>[2x]MKPEVEQELAHILLTELLAYQFASPVRWIETQDVFLKDFNTERVVEIGPSPTLAGMAQRTLKNKYESYDAALSLHREILCYSKDAKEIYYTPDPSELAAKEEPAKEEAPAPTPAASAPAPAAAAPAPVAAAAPAAAAAEIADEPVKASLLLHVLVAHKLKKSLDSIPMSKTIKDLVGGKSTVQNEILGDLGKEFGTTPEKPEETPLEELAETFQDTFSGALGKQSSSLLSRLISSKMPGGFTITVARKYLQTRWGLPSGRQDGVLLVALSNEPAARLGSEADAKAFLDSMAQKYASIVGVDLSSAASASGAAGAGAAAGAAMIDAGALEEITKDHKVLARQQLQVLARYLKMDLDNGERKFLKEKDTVAELQAQLDYLNAELGEFFVNGVATSFSRKKARTFDSSWNWAKQSLLSLYFEIIHGVLKNVDREVVSEAINIMNRSNDALIKFMEYHISNTDETKGENYQLVKTLGEQLIENCKQVLDVDPVYKDVAKPTGPKTAIDKNGNITYSEEPREKVRKLSQYVQEMALGGPITKESQPTIEEDLTRVYKAISAQADKQDISSSTRVEFEKLYSDLMKFLESSKEIDPSQTTQLAGMDVEDA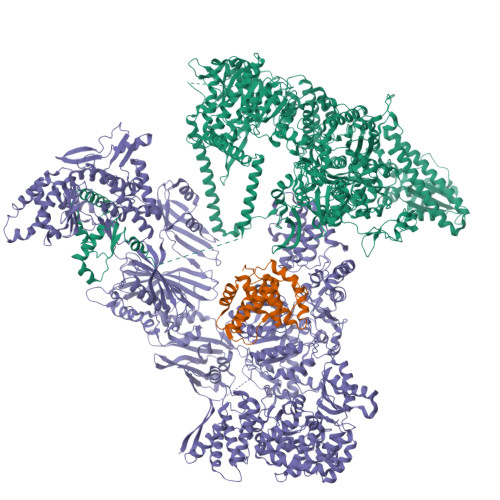LDKDSTKEVASLPNKSTISKTVSSTIPRETIPFLHLRKKTPAGDWKYDRQLSSLFLDGLEKAAFNGVTFKDKYVLITGAGKGSIGAEVLQGLLQGGAKVVVTTSRFSKQVTDYYQSIYAKYGAKGSTLIVVPFNQGSKQDVEALIEFIYDTEKNGGLGWDLDAIIPFAAIPEQGIELEHIDSKSEFAHRIMLTNILRMMGCVKKQKSARGIETRPAQVILPMSPNHGTFGGDGMYSESKLSLETLFNRWHSESWANQLTVCGAIIGWTRGTGLMSANNIIAEGIEKMGVRTFSQKEMAFNLLGLLTPEVVELCQKSPVMADLNGGLQFVPELKEFTAKLRKELVETSEVRKAVSIETALEHKVVNGNSADAAYAQVEIQPRANIQLDFPELKPYKQVKQIAPAELEGLLDLERVIVVTGFAEVGPWGSARTRWEMEAFGEFSLEGCVEMAWIMGFISYHNGNLKGRPYTGWVDSKTKEPVDDKDVKAKYETSILEHSGIRLIEPELFNGYNPEKKEMIQEVIVEEDLEPFEASKETAEQFKHQHGDKVDIFEIPETGEYSVKLLKGATLYIPKALRFDRLVAGQIPTGWNAKTYGISDDIISQVDPITLFVLVSVVEAFIASGITDPYEMYKYVHVSEVGNCSGSGMGGVSALRGMFKDRFKDEPVQNDILQESFINTMSAWVNMLLISSSGPIKTPVGACATSVESVDIGVETILSGKARICIVGGYDDFQEEGSFEFGNMKATSNTLEEFEHGRTPAEMSRPATTTRNGFMEAQGAGIQIIMQADLALKMGVPIYGIVAMAATATDKIGRSVPAPGKGILTTAREHHSSVKYASPNLNMKYRKRQLVTREAQIKDWVENELEALKLEAEEIPSEDQNEFLLERTREIHNEAESQLRAAQQQWGNDFYKRDPRIAPLRGALATYGLTIDDLGVASFHGTSTKANDKNESATINEMMKHLGRSEGNPVIGVFQKFLTGHPKGAAGAWMMNGALQILNSGIIPGNRNADNVDKILEQFEYVLYPSKTLKTDGVRAVSITSFGFGQKGGQAIVVHPDYLYGAITEDRYNEYVAKVSAREKSAYKFFHNGMIYNKLFVSKEHAPYTDELEEDVYLDPLARVSKDKKSGSLTFNSKNIQSKDSYINANTIETAKMIENMTKEKVSNGGVGVDVELITSINVENDTFIERNFTPQEIEYCSAQPSVQSSFAGTWSAKEAVFKSLGVKSLGGGAALKDIEIVRVNKNAPAVELHGNAKKAAEEAGVTDVKVSISHDDLQAVAVAVSTKK;> MDAYSTRPLTLSHGSLEHVLLVPTASFFIASQLQEQFNKILPEPTEGFAADDEPTTPAELVGKFLGYVSSLVEPSKVGQFDQVLNLCLTEFENCYLEGNDIHALAAKLLQENDTTLVKTKELIKNYITARIMAKRPFDKKSNSALFRAVGEGNAQLVAIFGGQGNTDDYFEELRDLYQTYHVLVGDLIKFSAETLSELIRTTLDAEKVFTQGLNILEWLENPSNTPDKDYLLSIPISCPLIGVIQLAHYVVTAKLLGFTPGELRSYLKGATGHSQGLVTAVAIAETDSWESFFVSVRKAITVLFFIGVRCYEAYPNTSLPPSILEDSLENNEGVPSPMLSISNLTQEQVQDYVNKTNSHLPAGKQVEISLVNGAKNLVVSGPPQSLYGLNLTLRKAKAPSGLDQSRIPFSERKLKFSNRFLPVASPFHSHLLVPASDLINKDLVKNNVSFNAKDIQIPVYDTFDGSDLRVLSGSISERIVDCIIRLPVKWETTTQFKATHILDFGPGGASGLGVLTHRNKDGTGVRVIVAGTLDINPDDDYGFKQEIFDVTSNGLKKNPNWLEEYHPKLIKNKSGKIFVETKFSKLIGRPPLLVPGMTPCTVSPDFVAATTNAGYTIELAGGGYFSAAGMTAAIDSVVSQIEKGSTFGINLIYVNPFMLQWGIPLIKELRSKGYPIQFLTIGAGVPSLEVASEYIETLGLKYLGLKPGSIDAISQVINIAKAHPNFPIALQWTGGRGGGHHSFEDAHTPMLQMYSKIRRHPNIMLIFGSGFGSADDTYPYLTGEWSTKFDYPPMPFDGFLFGSRVMIAKEVKTSPDAKKCIAACTGVPDDKWEQTYKKPTGGIVTVRSEMGEPIHKIATRGVMLWKEFDETIFNLPKNKLVPTLEAKRDYIISRLNADFQKPWFATVNGQARDLATMTYEEVAKRLVELMFIRSTNSWFDVTWRTFTGDFLRRVEERFTKSKTLSLIQSYSLLDKPDEAIEKVFNAYPAAREQFLNAQDIDHFLSMCQNPMQKPVPFVPVLDRRFEIFFKKDSLWQSEHLEAVVDQDVQRTCILHGPVAAQFTKVIDEPIKSIMDGIHDGHIKKLLHQYYGDDESKIPAVEYFGGESPVDVQSQVDSSSVSEDSAVFKATSSTDEESWFKALAGSEINWRHASFLCSFITQDKMFVSNPIRKVFKPSQGMVVEISNGNTSSKTVVTLSEPVQGELKPTVILKLLKENIIQMEMIENRTMDGKPVSLPLLYNFNPDNGFAPISEVMEDRNQRIKEMYWKLWIDEPFNLDFDPRDVIKGKDFEITAKEVYDFTHAVGNNCEDFVSRPDRTMLAPMDFAIVVGWRAIIKAIFPNTVDGDLLKLVHLSNGYKMIPGAKPLQVGDVVSTTAVIESVVNQPTGKIVDVVGTLSRNGKPVMEVTSSFFYRGNYTDFENTFQKTVEPVYQMHIKTSKDIAVLRSKEWFQLDDEDFDLLNKTLTFETETEVTFKNANIFSSVKCFGPIKVELPTKETVEIGIVDYEAGASHGNPVVDFLKRNGSTLEQKVNLENPIPIAVLDSYTPSTNEPYARVSGDLNPIHVSRHFASYANLPGTITHGMFSSASVRALIENWAADSVSSRVRGYTCQFVDMVLPNTALKTSIQHVGMINGRKLIKFETRNEDDVVVLTGEAEIEQPVTTFVFTGQGSQEQGMGMDLYKTSKAAQDVWNRADNHFKDTYGFSILDIVINNPVNLTIHFGGEKGKRIRENYSAMIFETIVDGKLKTEKIFKEINEHSTSYTFRSEKGLLSATQFTQPALTLMEKAAFEDLKSKGLIPADATFAGHSLGEYAALASLADVMSIESLVEVVFYRGMTMQVAVPRDELGRSNYGMIAINPGRVAASFSQEALQYVVERVGKRTGWLVEIVNYNVENQQYVAAGDLRALDTVTNVLNFIKLQKIDIIELQKSLSLEEVEGHLFEIIDEASKKSAVKPRPLKLERGFACIPLVGISVPFHSTYLMNGVKPFKSFLKKNIIKENVKVARLAGKYIPNLTAKPFQVTKEYFQDVYDLTGSEPIKEIIDNWEKYEQS>MKNFRLSEKEVKTLAKRIPTPFLVASLDKVEENYQFMRRHLPRAGVFYAMKANPTPEILSLLAGLGSHFDVASAGEMEILHELGVDGSQMIYANPVKDARGLKAAADYNVRRFTFDDPSEIDKMAKAVPGADVLVRIAVRNNKALVDLNTKFGAPVEEALDLLKAAQDAGLHAMGICFHVGSQSLSTAAYEEALLVARRLFDEAEEMGMHLTDLDIGGGFPVPDAKGLNVDLAAMMEAINKQIDRLFPDTAVWTEPGRYMCGTAVNLVTSVIGTKTRGEQPWYILDEGIYGCFSGIMYDHWTYPLHCFGKGNKKPSTFGGPSC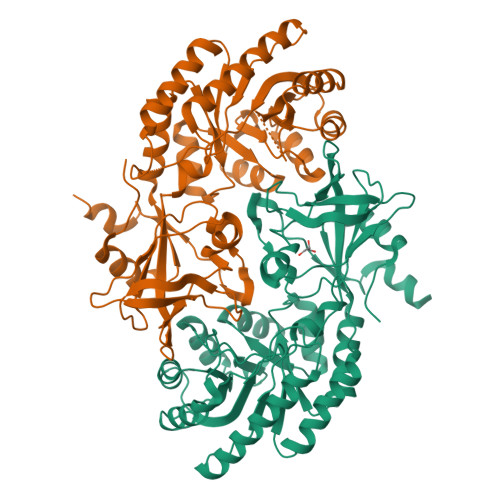DGIDVLYRDFMAPELKIGDKVLVTEMGSYTSVSATRFNGFYLAPTIIFEDQPEYAARLTEDDDVKKKAAV[2x]>[3x]SVLQVLHIPDERLRKVAKPVEEVNAEIQRIVDDMFETMYAEEGIGLAATQVDIHQRIIVIDVSENRDERLVLINPELLEKSGET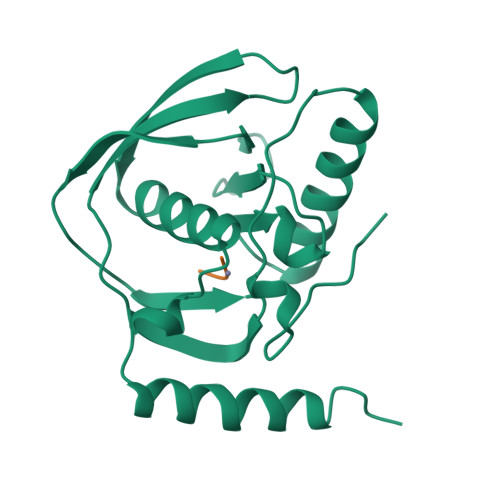GIEEGCLSIPEQRALVPRAEKVKIRALDRDGKPFELEADGLLAICIQHEMDHLVGKLFMDYLSPLKQQRIRQKVEKLDRLKARA;>[3x]MAS> MQVTHSMPPQKLEIFKSLDDWARNNVLIHLKSVEKSWQPQDYLPDPVSDGFEEQVRELRERAKEIPDDYFVVLVGDMITEEALPTYMSMLNRCDGIKDETGAEPSAWAMWTRAWTAEENRHGDLLN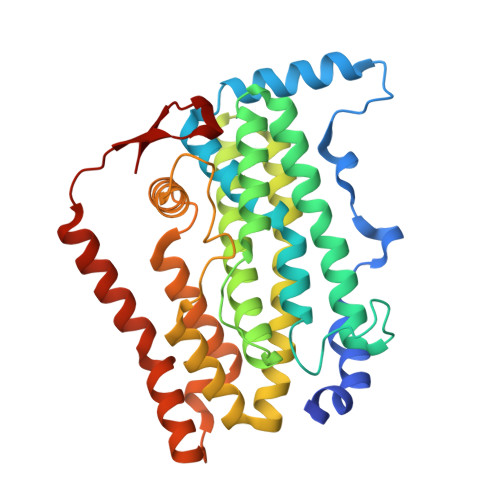KYLYLSGRVDMRKIEKTIQYLIGSGMDIKSENSPYLGFIYTSFQERATFISHANTAKLAQHYGDKKLAHICGSIASDEKRHATAYTKIVEKLAEIDPDTTVIAFADMMRKKITMPAHLMYDGSDELLFKHFTAVAQRLGVYSALDYCDILEFLVDKWNVERLTGLSDEGRKAQEYVCELGPKIRRLEERAQGRAKEAPTMPFSWIFDRQVKL> MGAQVSTEKSGSHETKNVATEGSTINFTNINYYKDSYAASASRQDFAQDPAKFTRPVLDTIREVAAPLQSPSVEACGYSDRVAQLTVGNSTITTQEAANIVLSYGEWPEYCPSTDATAVDKPTRPDVSVNRFYTLSTKSWKTESTGWYWKFPDVLNDTGVFGQNAQFHYLYRSGFCMHVQCNASKFHQGALLVAAIPEFVVAASSPATKPNGQGLYPDFAHTNPGKNGQEFRDPYVLDAGIPLSQALVFPHQWINLRTNNCATIIMPYVNALPFDSA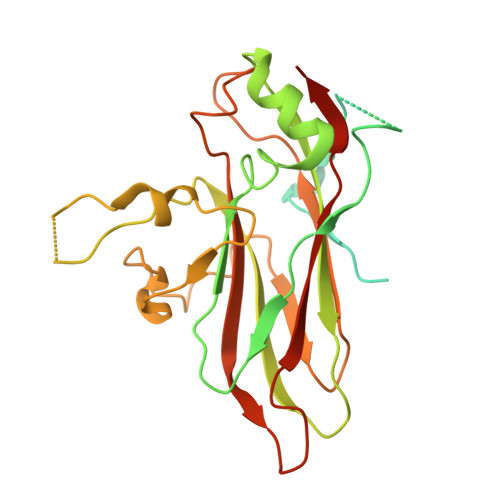LNHSNFGLVVIPISPLKYCNGATTEVPITLTIAPLNSEFSGLRQAIKQ>MGSDKIHHHHHHENLYFQGMINILVASEDASRLAHLARLVGDAGRYRVTRTVGRAAQIVQRTDGLDAFDILMIDGVALDTAELAAIEKLSRLHPGLTCMLVSADASSQTLLEAMRAGVRDVLR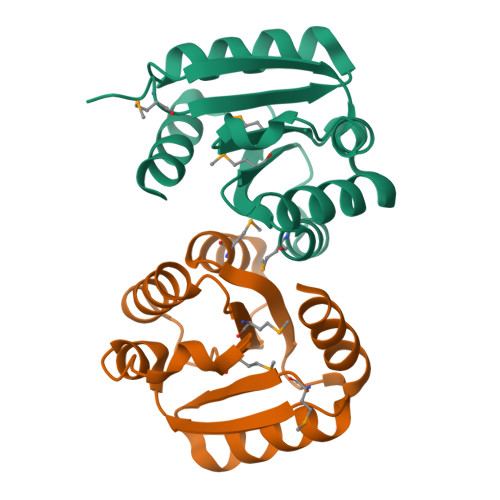WPLEPRALDDALKRAASQCAQRD[2x]> RAGPVTWVMMIACVVVFIAMQILGDQEVMLWLAWPFDPTLKFEFWRYFTHALMHFSLMHILFNLLWWWYLGGAVEKRLGSGKLIVITLISALLSGYVQQKFSGPWFGGLSGVVYALMGYVWLRGERDPQSGIYLQRGLIIFALIWIVAGWFDLFGMSMANGAHIAGLAVGLAMAFVDSL

Rhomboid intramembrane proteases are evolutionarily conserved proteins with numerous important biological functions, including growth factor secretion, regulation of mitochondrial dynamics, and membrane protein quality control (Fleig et al., 2012). Rhomboids are serine proteases with a Ser-His catalytic dyad (Wang et al., 2006), and they recognize their transmembrane substrates in a two-tier process. It is assumed that first a portion of the transmembrane domain of the substrate docks into an intramembrane interaction site of rhomboid within the plane of the lipid bilayer, upon which a linear segment of the substrate (possibly generated by local unfolding of the top of the substrate's transmembrane helix) interacts with the water-exposed active site (reviewed in Strisovsky, 2016a, Strisovsky, 2013).

To gain insight into these preferences and their possible interactions, we have generated tetra- and pentapeptidyl chloromethylketones (CMK or cmk henceforth) harboring amino acids preferred in positions P5 to P1 by the Escherichia coli rhomboid GlpG (GlpG henceforth), using the sequence background of the Providencia TatA (Stevenson et al., 2007), represented by the parent compound Ac-IATA-cmk. To provide mechanistic explanation for the observed increase in inhibitory potency, we determined the structures of GlpG in complex with Ac-RVRHA-cmk and Ac-VRHA-cmk. The side chain of Arg in the P5 position of Ac-RVRHA-cmk could not be modeled due to poor electron density, and the two structures are otherwise virtually identical; superposition of all corresponding Cα atoms yields a root-mean-square deviation of 0.19 Å per atom (using the SSM method as implemented in CCP4MG v2.10.4; Krissinel and Henrick, 2004, Mitchell et al., 1990). The interactions of the residues in the P4, P3, and P2 positions with the enzyme are structurally independent, explaining why the effects of substitutions in these positions are additive. The overall binding mode of both compounds into the rhomboid active site is similar to the binding mode of peptide aldehyde Ac-VRMA-cho (Cho et al., 2016). Collectively, these data show that rhomboid subsite preferences are additive in the context of an active site targeted inhibitor and that sequence optimization in this region can significantly increase the inhibitory potency of the compounds.>[2x]MALKYPSGKEYRGNKPNAARRPAADYANRGMTLEDDLNATNEYYRERGIAVIHKKPTPVQIVRVDYPKRSAAVITEAYFRQASTTDY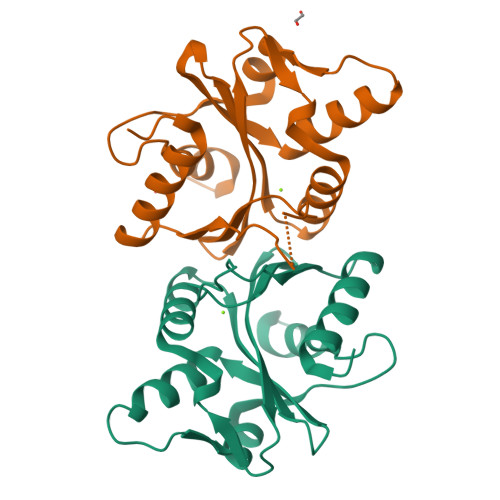NGVYRGKYIDFEAKETKNKTAFPLKNFHAHQIRHMEQVVAHGGICFAILRFSLLNETYLLDASHLIAWWNKQEAGGRKSIPKQEIERHGHSIPLGYQPRIDYISVVDNVYFTR> GPMTTTERPDLAWLDEVTMTQLERNPYEVYERLRAEAPLAFVPVLGSYVASTAEVCREVATSPDFEAVITPAGGRTFGHPAIIGVNGDIHADLRSMVEPALQPAEVDRWIDDLVRPIARRYLERFENDGHAELVAQYCEPVSVRSLGDLLGLQEVDSDKLREWFAKLNRSATNAAVDENGEFANPEGFAEGDQAKAEIRAVVDPLIDKWIEHPDDSAISHWLHDGMPPGQTRDREYIYPTIYVYLLGAMQEPGHGMASTLVGLFSRPEQLEEVVDDPTLIPRAIAEGLRWTSPIWSATARISTKPVTIAGVDLPAGTPV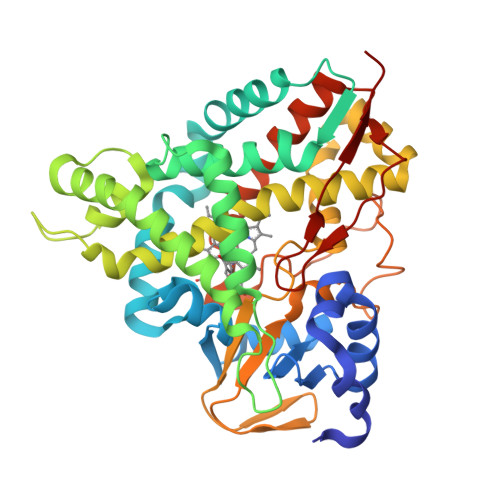MLSYGSANHDTGKYEAPSQYDLHRPPLPHLAFGAGNHACAGIYFANHVMRIALEELFEAIPNLERDTREGVEFWGWGFRGPTSLHVTWEV N-benzyl-3-{[(2Z,4S)-2-imino-4-methyl-6-oxo-4-(propan-2-yl)tetrahydropyrimidin-1(2H)-yl]methyl}benzamide 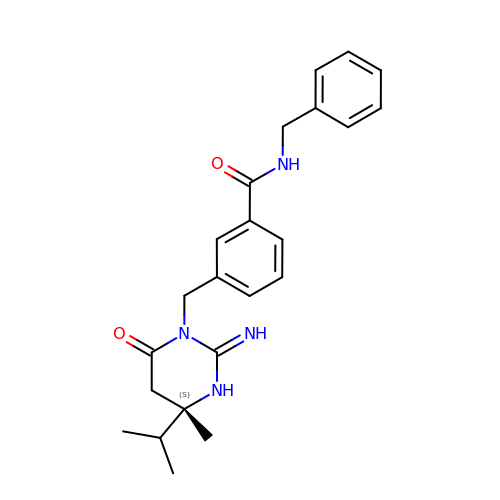| C23 H28 N4 O2 | OFTSPVADFMQIGQ-QHCPKHFHSA-N>[5x]MHCAENCIFCKIIAGDIPSAKVYEDEHVLAFLDISQVTKGHTLVIPKTHIENVYEF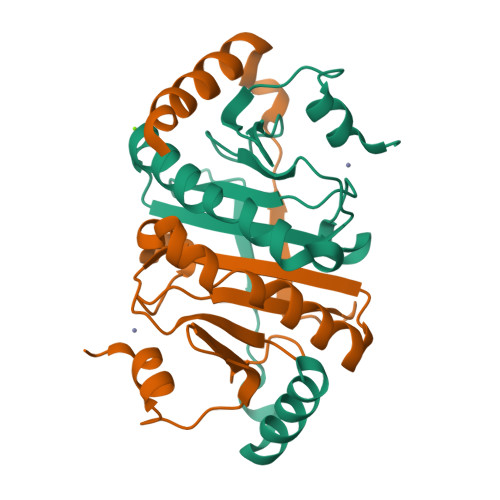TDELAKQYFHAVPKIARAIRDEFEPIGLNTLNNNGEKAGQSVFHYHMHIIPRYGKGDGFGAVWKTHADDYKPEDLQNISSSIAKRLASS>ADKLFINALKKKFEESPEEKKTTFYTLGGWKQSERKTEFVNAGKEVAAKRGIPQYNPDIGTPLGQRVLMPYQVSTTDTYVEGDDLHFVNNAAMQQMWDDIRRTVIVGLNHAHAVIEKRLGKEVTPETITHYLETVNHAMPGAAVVQEHMVETHPALVADSYVKVFTGNDEIADEIDPAFVIDINKQFPEDQAETLKAEVGDGIWQVVRIPTIVSRTCDGATTSRWSAMQIGMSMISAYKQAAGEAATGDFAYAAKHAEVIHMGTYLPVRRARGENEPGGVPFGYLADICQSSRVNYEDPVRVSLDVVATGAMLYDQIWLGSYMSGGVGFTQYATAAYTDNILDDFTYFGKEYVEDKYGLCEAPNNMDTVLDVATEVTFYGLEQYEEYPALLEDQFGGSQRAAVVAAAAGCSTAFATGNAQTGLSGWYLSMYLHKEQHSRLGFYGYDLQDQCGASNVFSIRGDEGLPLELRGPNYPNYAMNVGHQGEYAGISQAPHAARGDAFVFNPLVKIAFADDNLVFDFTNVRGEFAKGALREFEPAGERALITPAK[2x];>AKFEDKVDLYDDRGNLVEEQVPLEALSPLRNPAIKSIVQGIKRTVAVNLEGIENALKTAKVGGPACKIMGRELDLDIVGNAESIAAAAKEMIQVTEDDDTNVELLGGGKRALVQVPSARFDVAAEYSAAPLVTATAFVQAIINEFDVSMYDANMVKAAVLGRYPQSVEYMGANIATMLDIPQKLEGPGYALRNIMVNHVVAATLKNTLQAAALSTILEQTAMFEMGDAVGAFERMHLLGLAYQGMNADNLVFDLVKANGKEGTVGSVIADLVERALEDGVIKVEKELTDYKVYGTDDLAMWNAYAAAGLMAATMVNQGAARAAQGVSSTLLYYNDLIEFETGLPSVDFGKVEGTAVGFSFFSHSIYGGGGPGIFNGNHIVTRHSKGFAIPCVAAAMALDAGTQMFSPEATSGLIKEVFSQVDEFREPLKYVVEAAAEIKNEI[2x];>[2x]AQYYPGTTKVAQNRRNFCNPEYELEKLREISDEDVVKILGHRAPGEEYPSVHPPLEEMDEPEDAIREMVEPIDGAKAGDRVRYIQFTDSMYFAPAQPYVRSRA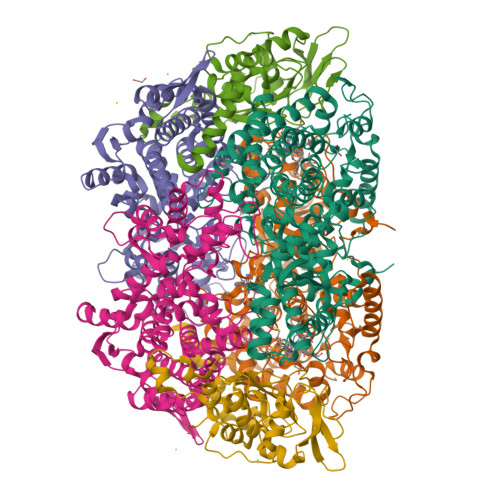YLCRYRGADAGTLSGRQIIETRERDLEKISKELLETEFFDPARSGVRGKSVHGHSLRLDEDGMMFDMLRRQIYNKDTGRVEMVKNQIGDELDEPVDLGEPLDEETLMEKTTIYRVDGEAYRDDVEAVEIMQRIHVLRSQGGFNLE> 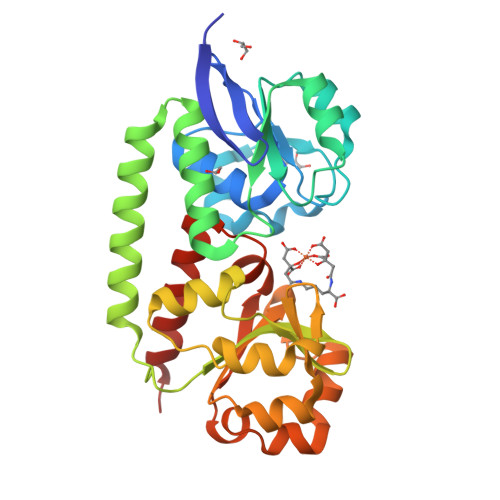GSHMASTISVKDENGTVKVPKDAKRIVVLEYSFADALAALDVKPVGIADDGKKKRIIKPVREKIGDYTSVGTRKQPNLEEISKLKPDLIIADSSRHKGINKELNKIAPTLSLKSFDGDYKQNINSFKTIAKALNKEKEGEKRLAEHDKLINKYKDEIKFDRNQKVLPAVVAKAGLLAHPNYSYVGQFLNELGFKNALSDDVTKGLSKYLKGPYLQLDTEHLADLNPERMIIMTDHAKKDSAEFKKLQEDATWKKLNAVKNNRVDIVDRDVWARSRGLISSEEMAKELVELSKKEQK> EAETRECIYYNANWELERTNQSGLERCEGEQDKRLHCYASWRNSSGTIEL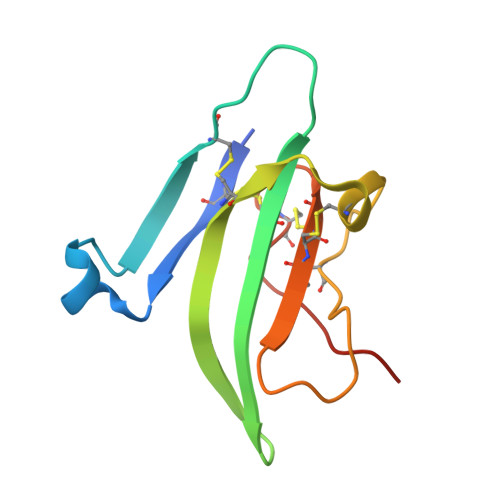VKKGCWLDDFNCYDRQECVATEENPQVYFCCCEGNFCNERFTHLPEPG>MGSSGKLADCTAQDLNRTELFLVEGDSAGGSAKQARDREYQAIMPLKGKILNTWEVSSDEVLASQEVHDISVAIGIDPDSDDLSQLRYGKICILADADSDGLHIATLLCALFVRHFRTLVKEGHVYVALPPLYRIDLGKEVYYALTEEEKTGVLEQLKRKKGKPNVQRFKGLGEMNPMQLRETTLDPNTRRLVQLVISDEDEQQTTAIMDMLLAKKRSE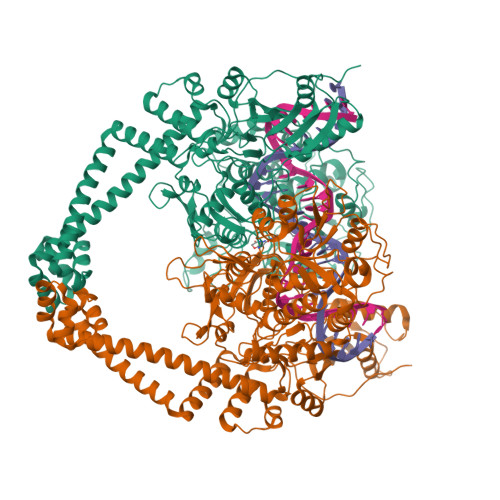DRRNWLQEKGDMADLEVESMSDMAERLALHEFTENAYLNYSMYVIMDRALPFIGDGLKPVQRRIVYAMSELGLNASAKFKKSARTVGDVLGKYHPHGDSACYEAMVLMAQPFSYRYPLVDGQGNWGAPDDPKSFAAMRYTESRLSKYAELLLSELGQGTVDWVPNFDGTLQEPKMLPARLPNILLNGTTGIAVGMATDIPPHNLREVAKAAITLIEQPKTTLDELLDIVQGPDFPTEAEIITSRAEIRKIYQNGRGSVRMRAVWSKEDGAVVISALPHQVSGAKVLEQIAAQMRNKKLPMVDDLRDESDHENPTRLVIVPRSNRVDMEQVMNHLFATTDLEKSYRINLNMIGLDGRPAVKNLLEILSEWLVFRRDTVRRRLNHRLEKVLKRLHILEGLLVAFLNIDEVIEIIRTEDEPKPALMSRFGISETQAEAILELKLRHLAKLEEMKIRGEQSELEKERDQLQAILASERKMNNLLKKELQADADAFGDDRRSPLHEREEAKALEHHHHHH[4x]> GGLPIVGDIFRFLDNGRTGLYENYKEFSTELNMTRESNGVKVTINDVISDGRTLSITYSLESEQDLG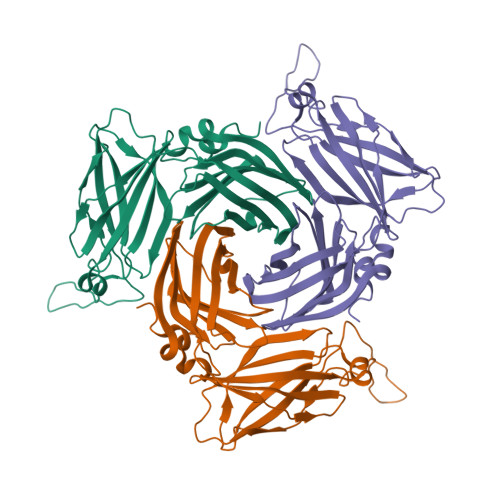DDPIILGGLDIMDAHGSSGSGKMTKVTEKKYVGMVTTTHHDSNKKDKVNFRWNIEGIEIPDRKKSIQGHWNFALTVKSMDSKERTIGGSSEKEGIKANMEKVAMSPVSFILYYNQEVSKGARKEWDSVDVELTVKDDLGNDYSGEGNGGSGNDPYNIRWSATFQKLNENATKLIVTPRVHLRVHTPENHGGVEYVNGKEKKIEVPNKEAKKKDIVLDDIVIDLKK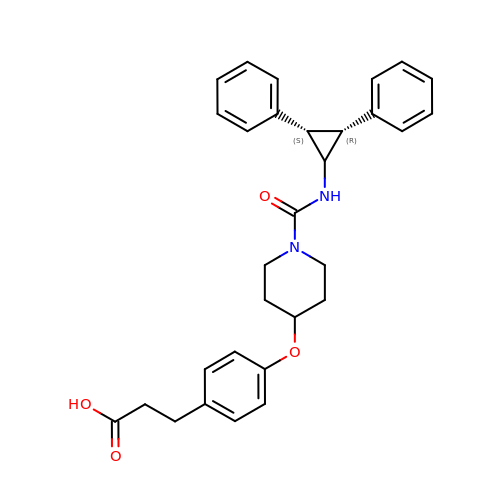3-{4-[(1-{[(1s,2R,3S)-2,3-diphenylcyclopropyl]carbamoyl}piperidin-4-yl)oxy]phenyl}propanoic acid | C30 H32 N2 O4 | VQQDJLMIDZHNMF-WLNZHLEZSA-N>SNAMDYQTIPSQGLSGEICVPGDKSISHRAVLLAAIAEGQTQVDGFLMGADNLAMVSALQQMGASIQVIEDENILVVEGVGMTGLQAPPEALDCGNSGTAIRLLSGLLAGQPFNTVLTGDSSLQRRPMKRIIDPLTLMGAKIDSTGNVPPLKIYGNPRLTGIHYQLPMASAQVKSCLLLAGLYARGKTCITEPAPSRDHTERLLKHFHYTLQKDKQSICVSGGGKLKANDISIPGDISSAAFFIVAATITPGSAIRLCRVGVNPTRLGVINLLKMMGADIEVTHYTEKNEEPTADITVRHARLKGID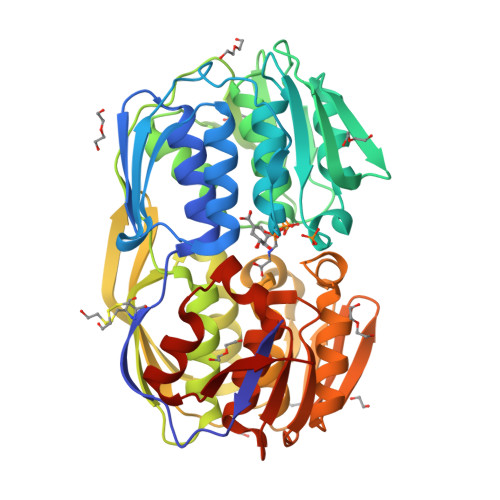IPPDQVPLTIDEFPVLLIAAAVAQGKTVLRDAAELRVKETDRIAAMVDGLQKLGIAAESLPDGVIIQGGTLEGGEVNSYDDHRIAMAFAVAGTLAKGPVRIRNCDNVKTSFPNFVELANEVGMNVKGVRGRGGF[4x]> MAIPAFHPGELNVYSAPGDVADVSRALRLTGRRVMLVPTMGALHEGHLALVRAAKRVPGSVVVVSIFVNPMQFGAGGDLDAYPRTPDDDLAQLRAEGVEIAFTPTTAAMYPDGLRTTVQPGPLAAELEGGPRPTHFAGVLTVVLKLLQIVRPDRV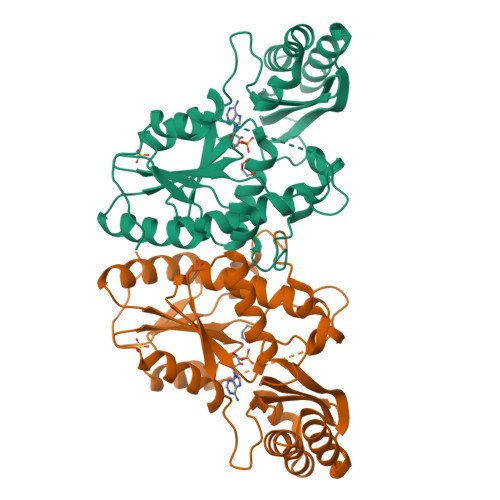FFGEKDYQQLVLIRQLVADFNLDVAVVGVPTVREADGLAMSSRNRYLDPAQRAAAVALSAALTAAAHAATAGAQAALDAARAVLDAAPGVAVDYLELRDIGLGPMPLNGSGRLLVAARLGTTRLLDNIAIEIGTFAGTDRPDGYR[6-methyl-5-oxidanyl-4-[(~{E})-[(1~{R})-1-phenylethyl]iminomethyl]pyridin-3-yl]methyl 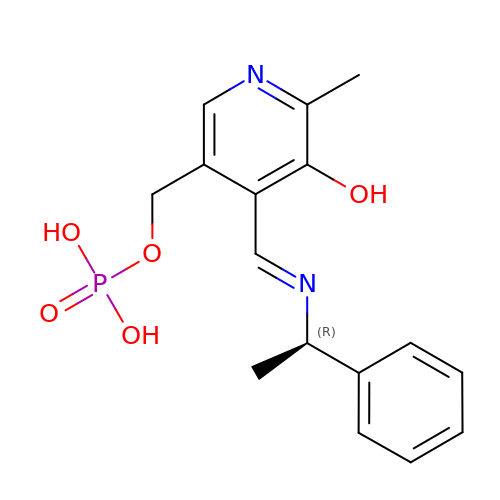dihydrogen phosphate | C16 H19 N2 O5 P | ZBWJIKYNMPWLJE-PBFYJAPKSA-N(2R,3aR,5R,6R,7R,7aR)-5-(hydroxymethyl)-2-methylhexahydro-3aH-pyrano[3,2-d][1,3]thiazole-6,7-diol 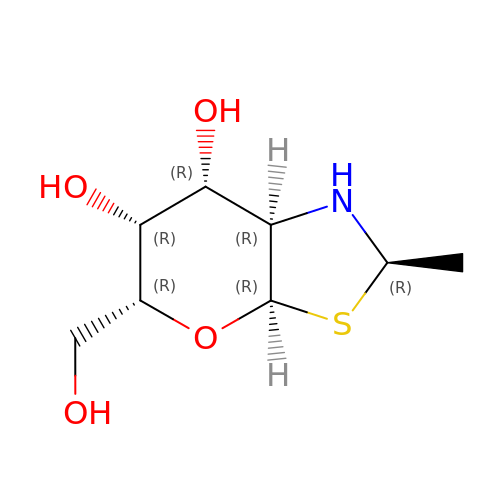| C8 H15 N O4 S | XWPUWEBFKDEDIF-CVBHLRHXSA-N> MLEARFQQAALLKKLLDAIKELVTDANFDCNDNGISLQAMDSSHVALVSMLIKSDGFEPYRCDRNIALGINLNALSKVLRCAQNEDLVTLKAEDTPEVLNLVFESEKNDRISDYDVKLMDI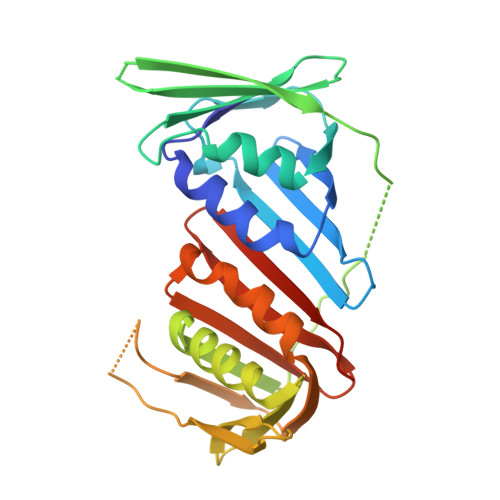DQEHLGIPDIEYDATITMPAAEFQRITRDLLTLSDSVTINASKEGVRFSCKGDIGNGSTTLKQHTDLSDQDQSIEISLTQAVTLTFSLKYLAQFTKATPLATRVTLSMSNDVPLLVEYKMESGFLRFYLAPKIGEEDEE> TAKNTVVRGLENVEALEGGEALFECQLSQPEVAAHTWLLDDEPVRTSENAEVVFFENGLRHLLLLKNLRPQDSCRVT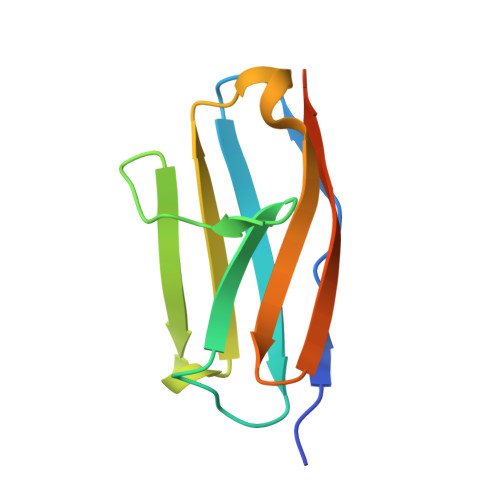FLAGDMVTSAFLTVRGGLEHHHHHH> CVAVEQKTRTAIIRIGTRGSPLALAQAYETREKLKKKHPELVEDGAIHIEIIKTTGDKILSQPLADIGGKGLFTKEIDEALINGHIDIAVHSMKDVPTYLPEKTILPCNLPREDVRDAF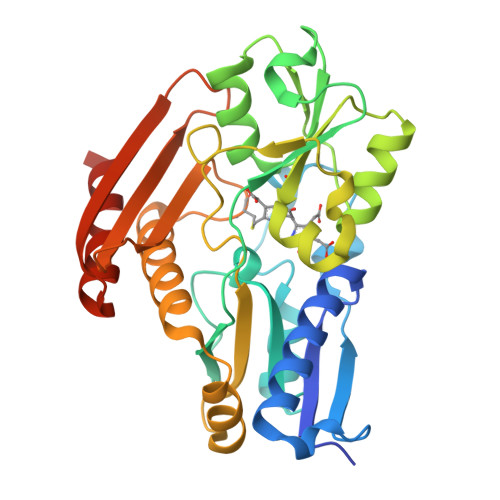ICLTAATLAELPAGSVVGTASLRRKSQILHKYPALHVEENFRGNVQTRLSKLQGGKVQATLLALAGLKRLSMTENVASILSLDEMLPAVAQGAIGIACRTDDDKMATYLASLNHEETRLAISCERAFLETLDGSCRTPIAGYASKDEEGNCIFRGLVASPDGTKVLETSRKGPYVYEDMVKMGKDAGQELLSRAGPGFFGN>[7x]MHHLLEQSADMATALLAGEKLRELILPG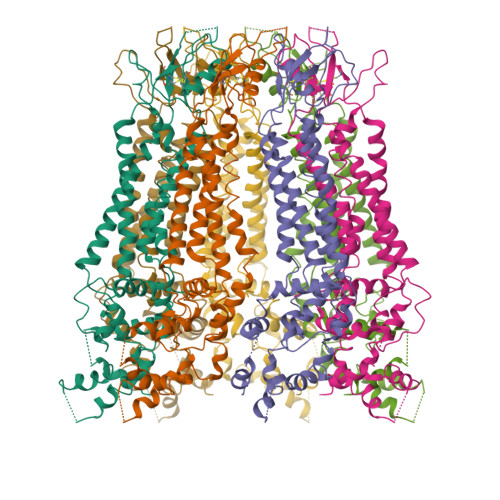AQDDKAGALAALLLQLKLELPFDRVVTIGTVLVPILLVTLVFTKNFAEEPIYCYTPHNFTRDQALYARGYCWTELRDALPGVDASLWPSLFEHKFLPYALLAFAAIMYVPALGWEFLASTRLTSELNFLLQEIDNCYHRAAEGRAPKIEKQIQSKGPGITEREKREIIENAEKEKSPEQNLFEKYLERRGRSNFLAKLYLARHVLILLLSAVPISYLCTYYATQKQNEFTCALGASPDGAAGAGPAVRVSCKLPSVQLQRIIAGVDIVLLCVMNLIILVNLIHLFIFRKSNFIFDKLHKVGIKTRRQWRRSQFCDINILAMFCNENRDHIKSLNRLDFITNESDLMYDNVVRQLLAALAQSNHDATPTVRDSGVQTVDPSAN>[4x]MGSHHHHHHGRSMSELIKENMHMKLYMEGTVNNHHFKCTSEGEGKPYEGTQTMRIKVVEGGPLPFAFDILATSFMYGS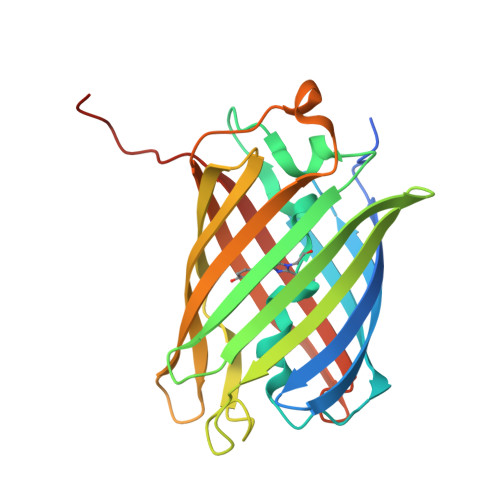YTFINHTQGIPDFFKQSFPEGFTWERVTTYEDGGVLTATQDTSLQDGCLIYNVKIRGVNFTSNGPVMQKKTLGWEAGTEMLYPADGGLEGRSDEALKLVGGGHLICNLKSTYRSKKPAKNLKVPGVYYVDRRLERIKEADKETYVEQHEVAVARYCDLPSKLGHKLN>[2x]RRHTLPANEFRCLTPEDAAGVFEIEREAFISVSGNCPLNLDEVQHFLTLCPELSLGWFVEGRLVAFIIGSLWDEER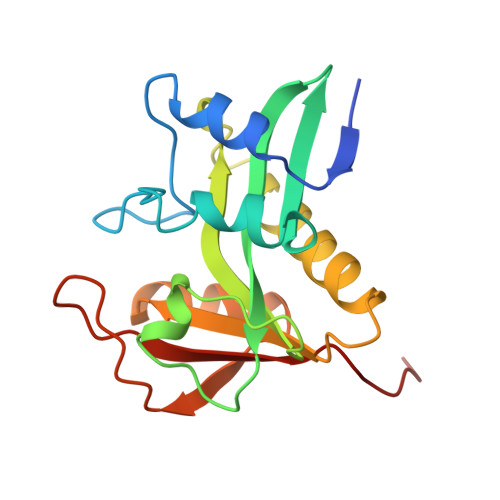LTQESLALHRPRGHSAHLHALAVHRSFRQQGKGSVLLWRYLHHVGAQPAVRRAVLMCEDALVPFYQRFGFHPAGPCAIVVGSLTFTEMHCSLRGHAAL> MPYSVGFREADAATSFLRAARSGNLDKALDHLRNGVDINTCNQNGLNGLHLASKEGHVKMVVELLHKEIILETTTKKGNTALHIAALAGQDEVVRELVNYGANVNAQSQKGFTPLYMAAQENHLE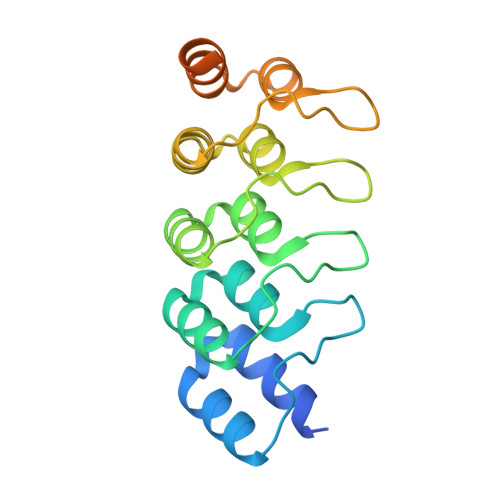VVKFLLENGANQNVATEDGFTPLAVALQQGHENVVAHLINYGTKGKVRLPALHIAARNDDTRTAAVLLQNDPNPDV>[2x]ERVNVNLTSIKKLREKVDDSIHRELTDIFANLNYVGVVDEERRLAAIQHDLKLFLIDYGSVCYELFYQIGLTDFANFGKINLQSTNVSDDIVLYNLLSEFDELNDDASKEKIISKIWDMSSMLNEYY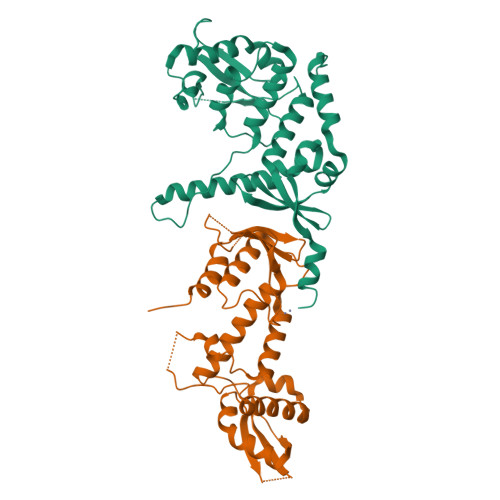SIELVNDGLDNDLKSVKLKSLPLLLKGYIPSLVKLPFFIYRLGKEVDWEDEQECLDGILREIALLYIPDMVPKVDTSDASLSEDEKAQFINRKEHISSLLEHVLFPCIKRRFLAPRHILKDVVEIANLPDLYKVFERC;>[2x]GKTITDFSISRSVLAKYEVINQVDKKFILIRCLDQSIHNCPLLVLVDQHACDERIRLEELFYSLLTEVVTGTFVARDLKDCCIEVDRTEADLFKHYQSEFKKWGIGYETIEGTMETSLLEIKTLPEMLTSKYNGDKDYLKMVLLQHAHDLKDFKKLPMDLSHFENYTSVDKLYWWKYSSCVPTVFHEILNSKACRSAVMFGDELTRQECIILISKLSRCHNPFECAHGRPSMVPIAELK>[2x]AANDNNVEWNGLFHDQGPLFDNAPEPTSTQSVTLKLRTFKGDITSANIKYWDTADNAFHWVPMVWDSNDPTGTFDYWKGTIP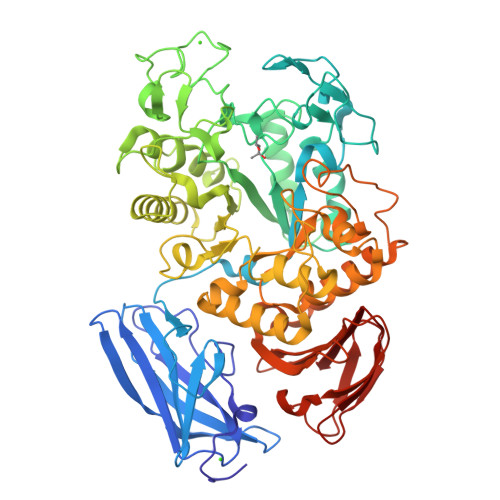ASPSIKYYRFQINDGTSTAWYNGNGPSSTEPNADDFYIIPNFKTPDWLKNGVMYQIFPDRFYNGDSSNDVQTGSYTYNGTPTEKKAWGSSVYADPGYDNSLVFFGGDLAGIDQKLGYIKKTLGANILYLNPIFKAPTNHKYDTQDYMAVDPAFGDNSTLQTLINDIHSTANGPKGYLILDGVFNHTGDSHPWFDKYNNFSSQGAYESQSSPWYNYYTFYTWPDSYASFLGFNSLPKLNYGNSGSAVRGVIYNNSNSVAKTYLNPPYSVDGWRLDVANEVDANGNNGSDVTNHQIWSEFRNAVKGVNSNAAIIGEYWGNANPWTAQGNQWDAATNFDGFTQPVSEWITGKDYQNNSASISTTQFDSWLRGTRANYPTNVQQSMMNFLSNHDITRFATRSGGDLWKTYLALIFQMTYVGTPTIYYGDEYGMQGGADPDNRRSFDWSQATPSNSAVALTQKLITIRNQYPALRTGSFMTLITDDTNKIYSYGRFDNVNRIAVVLNNDSVSHTVNVPVWQLSMPNGSTVTDKITGHSYTVQNGMVTVAVDGHYGAVLAQ> MGSSHHHHHHSQDPMEIDELTALGGLLHDIGKPVQRAGLYSGDHSTQGARFLRDLAENTGRAEYELLSLFSEFHHKGHMKNDELMIRRIKELSPERFGLTMEDVLNALWIVYEADNLASGEREEGQPQASRPLYSVFNPGKAYPWAELDFEKELPVPGDVFSIRSQDYRELVKRLWEELSKAKLRSDRLLPVLEKYLTFVSSVTSEGNIISLYDHMRMTSAIALAMLRAGCTAEDVRSGRCRKEKRFLLIEGDFSGIQDFIYRVSGKGTLKYLRARSAYLELIGWDVVLEILSRLGLTRANVVFNAGGHFMIIAQNTPDAVKELEEIRAKAVEWLYREFESDLYLAIEWEPVSGREFGREGGKNLFAEARKRLKHKLTVRKLKRFGEIKGLFEHGHTERLAECPVCGRELPEGKLEPSASDPETKVCPTCNRLVSLGGNLPKLLGFGRTAKNDAGVLVEGPFSGFVPYLQGGRPVGEQILVKNTLNPGEIPESAQFVPYFVADYFKKDPKGGVATFEELSMASTGTRRLGVMKGDVDRLGEFFSSMDSPSKLATASRFMDYFFKGYIGAIIEGKFGYIIGDVPSLRDWPEEPDIVVVYAGGDDFFIVGAWDQIFELAFRVRRAFNAYTGGKLTLSVGLGYFDERTPIYRMADVVSERLDTAKDEGRNRVFVVGRSRPLDGKHKLSYEWNHYEELWRTYAPRIYAGNGRLKGKLESKKGLLWKLLEIRELYVRDPNDVRWAYLTAYLLGRHGLSDLFPELVGIDTKAVERKEPQPVYWVDGVLKIVLMAVRR;> SMAYHQKHGGYGRGGYGRQDRPQVDASRLFGESPDVVGIKKMLEGKGKQWEAIQPYFDNVVREAKNFLEWSPNKRLANAVTVAAYLTSQGLKTNQVRKILDMARTTELKVKRGEGDIKDDLVKMRYLLAYTVGKATGQSKYSLDAFHRILDPMLEVLMGSPKKENFEKFYDFLQAVVAYHKFFGGGD;>SMDRRFYGKIVIKGKIKAVTGLHIGSQRDISEIGGIDNPVIKDPHTGLPYIPGSSLKGRLRSLFEILVNSRLGEWREKYPSLANYSPGSCRPDNQENCGKFFNRKINRGWIHVCPDYETALACPVCRLFGASGKESNFPSRIIVRDAFLTKEWEEKWRAGEAITEAKIEVGIDRVTSQANPRTNERVVAGAEFEFEIIYNVENTTHWRDDIKNLLTAMALLEDSYLGGSGSRGYGKVKFIFDSFEFRPLDYYRTGKDEDIVSIDAREKSVSDILSGFDSLFSEVEGKLEAG[2x];> MPKFIAVKLIPKGPFRDIPRADTLFGAIGNAISAIHGQSAVEELVDAFVGGARISSAFPYSGDTYYLPKPLSVEPALEGILTGLDEEERYTTAKRLRKAKYLDLKNFELALRLRPFTIPEEIPYARVDVPRVVLDRVTQDSSIYFWEEIRFREKSGVYFLYSGPREVFDGYIAPAMRFLGDTGIGGKSTWGAGLFEVEFHEMKIDAPGSEYSVTLSNALPTKTPVLWRLLRKGGWSFGRRKPRMTFIAEGSIVKNDPGGMERLELGLSHEVYVYGLTFPLGVELPEGLE;> MTERTLKVLSPLHIGTGNELTPVDIYPRENIIHVLDTERLVNDLMNLGVELNEILALLKNPPGDAYIWKGYIEEFHLDPSDYSIYTLKIHGKIGRKSMQIKEFIKLNGRPYIPGSSLKGAIRTAVLYKALKECGDARAVMRVVSKVNGDVARDIGRSEDVLDYYMSFLSRARIDRKRADDLLEAIVFGMEPDRRSKIRYEPKRDPMKALIVRDSKPVGRKHLAVYHVEVIGNPQPIPIWVEAIEPGAATDVEIHVDTEALRLNADYFNGLLWECLKERGEPGEVFEDFLWEAVDEFYTAVMKYETIEVQKFGRYTSQVRSFYASLEDHSGHVLRLGWGSGWLAMTIGLLLVEKGYKWENVRKKLGLGKKPGGSGFSREFPKTRRLADGMPMGWVVLEHHHH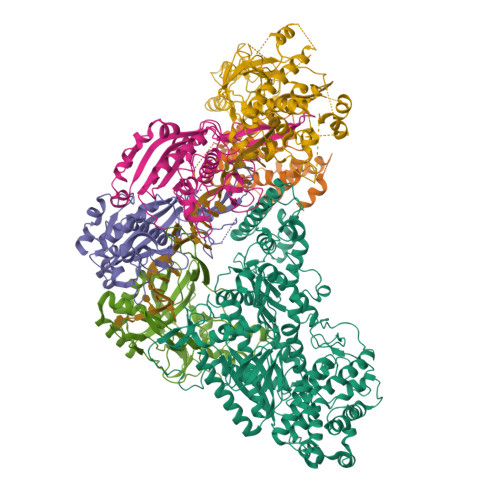HH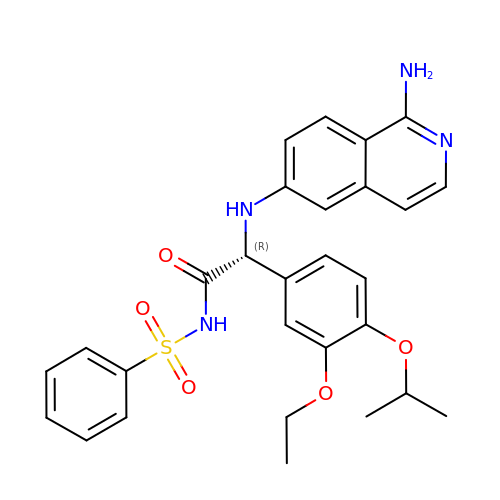(2R)-2-[(1-aminoisoquinolin-6-yl)amino]-2-[3-ethoxy-4-(propan-2-yloxy)phenyl]-N-(phenylsulfonyl)ethanamide | C28 H30 N4 O5 S | ICZUITMFGXCICW-AREMUKBSSA-N> GSKFSSDASKVVTRGPGLSQAFVGQKNSFTVDCSKAGTNMMMVGVHGPKTPCEEVYVKHMGNRVYNVTYTVKEKGDYILIVKWGDESVPGSPFKVKVP;> GSGNIKTLGDAYEFAVDVRDFSPEDIIVTTSNNHIEVRAEKLAADGTVMNTFAHKSQLPEDVDPTSVTSALREDGSLTIRARRHPHT

HSPB7 is a member of the small Heat-Shock Protein (sHSP) family, and is expressed specifically in heart and skeletal muscle. Though it shares the common architecture of sHSPs (an α-crystallin domain, ACD, flanked by N- and C-terminal regions), HSPB7 is unusual as it has been observed to be oligomerisation incompetent. FLNC interacts with HSPB7, also known as cardiovascular heat-shock protein (cvHSP), via d2417–20. Our work therefore shows, structurally, how HSPB7 acts as a specific molecular chaperone that regulates FLNC dimerisation.

Given the nature of the heterodimer between HSPB7ACD and FLNCd24 as composed of two well-structured units interacting with nanomolar affinity, we considered them a strong candidate for co-crystallisation. We were successful in obtaining crystals of the complex, which diffracted to 2.9 Å, and solved the structure in the P3221 space group. The asymmetric unit comprised a single heterodimer, with the interface centred around a parallel pairing of FLNCd24 strand C with HSPB7ACDC131S β4, and the donation of sidechains from each strand into an adjacent hydrophobic groove on each monomer (β4-β8 groove on HSPB7ACD, and C-D groove on FLNCd24). Note that this is a different site and mode of association to that observed in the dimerisation of sHSP ACDs, which occurs via anti-parallel pairing of β6 + 7 strands. Specifically, the HSPB7 β4-β8 groove accepts M2667 and M2669 from FLNC, while the groove between strands C and D accepts I102. The interface is thus mainly comprised of hydrophobic contacts made between the monomers’ sidechains, with additional stability conferred by polar contacts between the chains. The protection measured between HSPB7 β3 and β4 (residues 90–100) can be rationalised by the salt bridge formed between D100 and FLNC H2686. We assayed the strength of this interaction quantitatively for HSPB7ΔN and HSPB7ACD by performing experiments at a range of FLNCd24 concentrations; the instability of full-length HSPB7 (some unfolding is observed in the native MS spectra, and we found the protein could readily precipitate in vitro) precluded reliable equivalent experiments for it. This allowed us to obtain dissociation constants (KD) for the FLNCd24:HSPB7ΔN heterodimer as 6.7 ± 1.4 nM and FLNCd24:HSPB7ACD heterodimer as 3.9 ± 0.9 nM, significantly tighter binding than we measured for the FLNCd24 homodimer (75.9 ± 8.4 nM), by >6 kJmol-1 (see later). Bearing in mind that HDX-MS operates at a resolution defined by the enzymatic digestion (and hence unaffected residues can appear protected simply by being within the same peptide product as residues that truly are), mapping the protection from deuteration measured onto our structure emphasises how protection is highest near the crystallographically observed interface. This also shows that the C131S mutation that we introduced to aid crystallisation, but was absent in the construct used in HDX-MS, does not alter the location of the dimer interface.>MTNTDLKPLLDNLRNATEFWNLVKEASATDESTVHNRSYRDALDWLESAALALGDALIAQRKAVGGDHE[4x];>[2x]MALVDGFLELERSSGKLEWSAILQKMASDLGFSKILFGLLPKDSQDYENAFIVGNYPAAWREHYDRAGYARVDPTVSHCTQSVLPIFWEPSIYQTRKQHEFFEEASAAGLVYGLTMPLHGARGELGALSLSVEAENRAEANRFMESVLPTLWMLKDYALQSGAGLAFEHPVSKPVVLTSREKEVLQWCAIGKTSWEISVICNCSE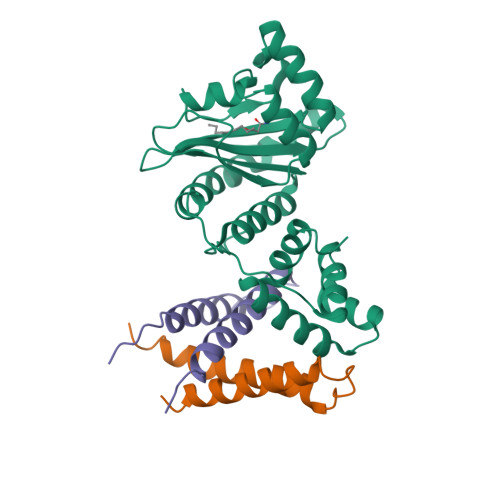ANVNFHMGNIRRKFGVTSRRVAAIMAVNLGLITL>[2x]IQTTAPPVKESSFVEKMKKTGRNIIVFYGSQTGTAEEFANRLSKDAHRYGMRGMSADPEEYDLADLSSLPEIDKSLVVFCMATYGEGDPTDNAQDFYDWLQETDVDLTGVKFAVFGLGNKTYEHFNAMGKYVDQRLEQLGAQRIFELGLGDDDGNLEEDFITWRE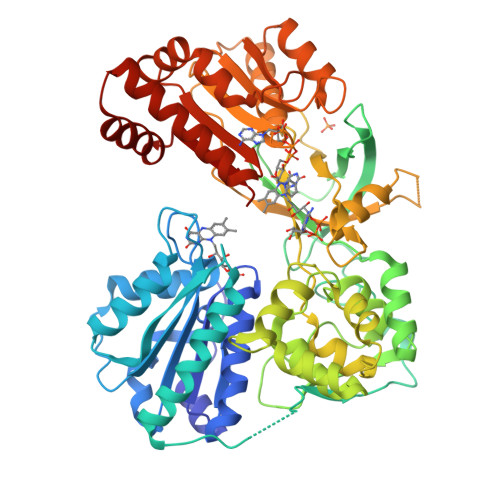QFWPAVCEFFGVEATGEESSIRQYELVVHEDMDVAKVYTGEMGRLKSYENQKPPFDAKNPFLAAVTANRKLNQGTERHLMHLELDISDSKIRYESGDHVAVYPANDSALVNQIGEILGADLDVIMSLNNLDEESNKKHPFPCPTTYRTALTYYLDITNPPRTNVLYELAQYASEPSEQEHLHKMASSSGEGKELYLSWVVEARRHILAILQDYPSLRPPIDHLCELLPRLQARYYSIASSSKVHPNSVHICAVAVEYEAKSGRVNKGVATSWLRAKEPAGENGGRALVPMFVRKSQFRLPFKSTTPVIMVGPGTGIAPFMGFIQERAWLREQGKEVGETLLYYGCRRSDEDYLYREELARFHKDGALTQLNVAFSREQAHKVYVQHLLKRDREHLWKLIHEGGAHIYVCGFARNMAKDVQNTFYDIVAEFGPMEHTQAVDYVKKLMTKGRYSLDVWS>MAHHHHHHMDLGIAGKTALVCAASKGLGRGCAEALAAEGVNLVIVARTRDTLERTADEIRAASNVSVATVACDITTPDGRAA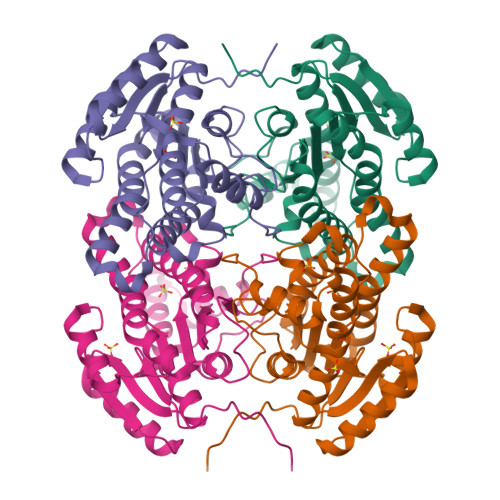ALAACPQPDILVNNAGGPPPGDFRDFSHDDWIRALESNMLTPIELIRATVDGMIARGFGRIVNITSSAVKAPIDVLALSNGARSGLTGFVAGLARKVVGQGVTINNLLPGLFDTDRIATTLAAAANAQGVTVDELRARRTRDIPAGRLGTRAEFGAACAFLCSVHAGYITGQNWLLDGGAYPGTF[2x]1-METHYL-2-(2-{[5-(4-METHYLPIPERAZIN-1-YL)-2-(TRIFLUOROMETHOXY)PHENYL]AMINO}PYRIMIDIN-4-YL)-1,5,6,7-TETRAHYDRO-4H-PYRROLO[3,2-C]PYRIDIN-4-ONE 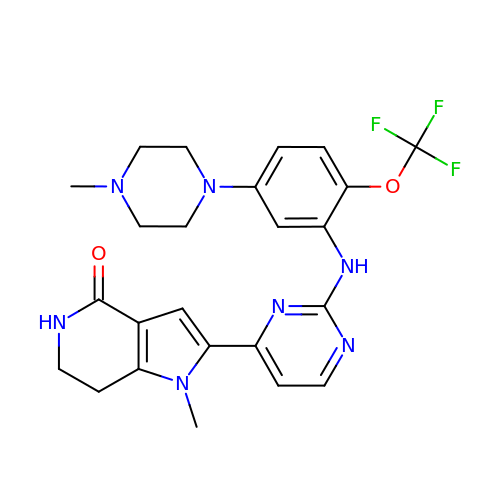| C24 H26 F3 N7 O2 | CYXABCVHENZAID-UHFFFAOYSA-N> MLERRPMAQVFDRRANTLARVSIFAGIPLVLAILGGVWWLFGWSDWHRDVGVEIPQPGGGFNHQLHVALGMDCRYCHTAVEVSAHANIPPTETCMGCHSQIISRSEKVAFVWQSWETGTSIQWNKVHDLPKFVYFNHSIHVAKGVGCSTCHGRIDQMRVVYKTQPLFMSWCLDCHRNPEKYVRPREEVFNMAWTPPPNQLEVGRRLVQEYEIRSSWE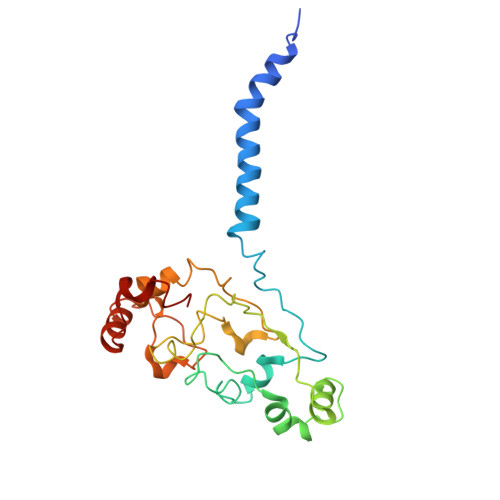LTNCAICHR> EEGLDFPEYDGVDRVVNVNAKNYKNVFKKYEVLALLYHEPPEDDKASQRQFEMDELILELAAQVLEDKGVGFGMVDSEKDAAVAKKLGLTEEDSVYVFKGDEVIEYDGEFSADTLVEFL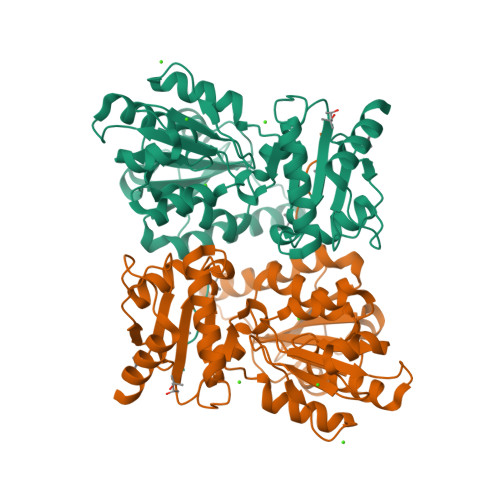LDVLEDPVELIEGERELQAFENIEDDNKLIGYFKNKDSEHYKAYEDAAEEFHPYIPFFATFDSKVAKKLTLKLNEIDFYEAFMEEPVTIPDKPNSEEEIVSFVEAHKRSTLRKLKPESMYETWEDDLDGIHIVAFAEETDPDGYEFLETLKAVAQDNTDNPDLSIIWIDPDDFPLLVPYWEKTFNIDLSAPQIGVVNVTDADSVWMEMDDEEDLPSAEELEDWLEDVLEGEINTEDDDEEDD> ISPIETVPVKLKPGMDGPKVKQWPLTEEKIKALVEICTEMEKEGKISKIGPENPYNTPVFAIKKKDSTKWRKLVDFRELNKRTQDFWEVQLGIPHPAGLEKKKSVTVLDVGDAYFSVPLDEDFRKYTAFTIPSINNETPGIRYQYNVLPQGWKGSPAIFQSSMTKILEPFRKQNPDIVIYQYMDDLYVGSDLEIGQHRTKIEELRQHLLRWGLTTPDKKHQKEPPFLWMGYELHPDKWTVQPIVLPEKDSWTVNDIQKLVGKLNWASQIYPGIKVRQLCKLLRGTKALTEVIPLTEEAELELAENREILKEPVHGVYYDPSKDLIAEIQKQGQGQWTYQIYQEPFKNLKTGKYARMRGAHTNDVKQLTEAVQKITTESIVIWGKTPKFKLPIQKETWETWWTEYWQATWIPEWEFVNTPPLVKLWYQLEKEPIVGAETFYVDGAANRETKLGKAGYVTNRGRQKVVTLTDTTNQKTELQAIYLALQDSGLEVNIVTDSQYALGIIQAQPDQSESELVNQIIEQLIKKEKVYLAWVPAHKGIGGNEQV;> ETVPVKLKPGMDGPKVKQWPLTEEKIKALVEICTEMEKEGKISKIGPENPYNTPVFAIKKKDSTKWRKLVDFRELNKRTQDFWEVQLGIPHPAGLEKKKSVTVLDVGDAYFSVPLDEDFRKYTAFTIPSINNETPGIRYQYNVLPQGWKGSPAIFQSSMTKILEPFRKQNPDIVIYQYMDDLYVGSDLEIGQHRTKIEELRQHLLRWGLTTPDKKHQKEPPFLWMGYELHPDKWTVQPIVLP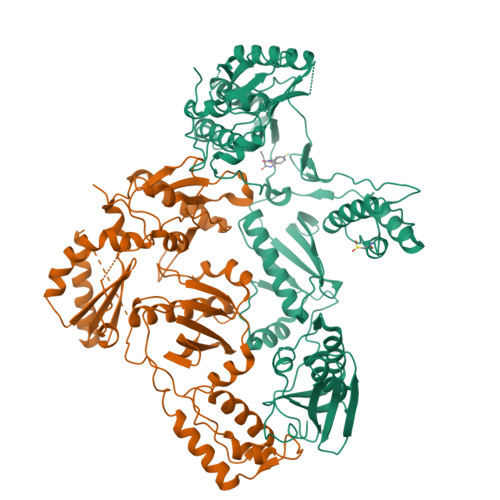EKDSWTVNDIQKLVGKLNWASQIYPGIKVRQLCKLLRGTKALTEVIPLTEEAELELAENREILKEPVHGVYYDPSKDLIAEIQKQGQGQWTYQIYQEPFKNLKTGKYARMRGAHTNDVKQLTEAVQKITTESIVIWGKTPKFKLPIQKETWETWWTEYWQATWIPEWEFVNTPPLVKLWYQLEK> MGSSHHHHHHSSGLVPAGSHMAGTKKGVSAAAFSGVTAALGDVGARWFYTWAADPQGITAPAGTEFVPMIWGRDSVTADQLQRAKAAGSTLLAFNEPDLAGQANMS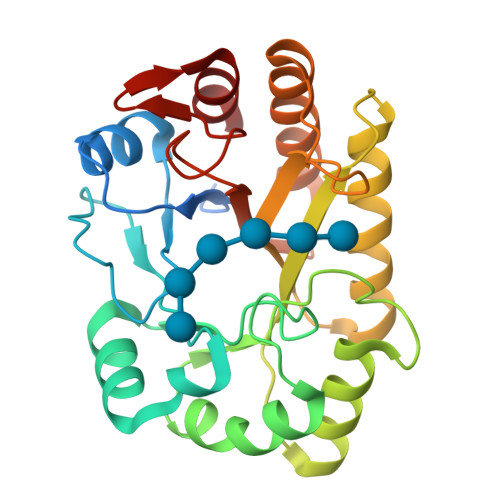VETALDLWPQLQATGMRLGAPAVAYGGDTPGGWLDRFMSGAAARGYRVDFIPLHWYGGDFSAAATGQLQSYLQAVYNRYHRPIWLTQYALTDFSGSTPRYPSAAEQADFVSRSTAMLNGLSFVERYAWFSLSTSTTPTGLYTGTTPNSSGVAYRAAG>[2x]TIKVGINGFGRIGRIVFRAAQKRSDIEIVAINDLLDADYMAYMLKYDSTHGRFDGTVEVKDGHLIVNGKKIRVTAERDPANLKWDEVGVDVVAEATGLFLTDETARKHITAGAKK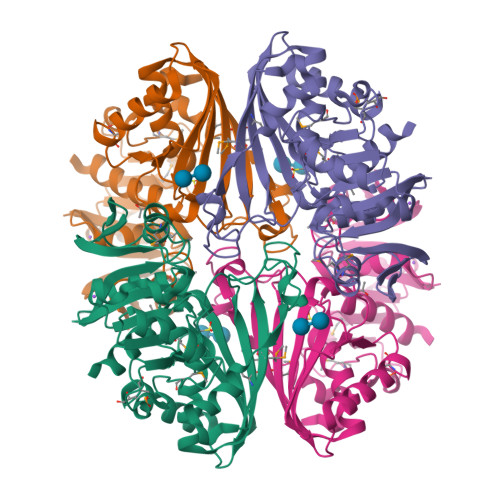VVMTGPSKDNTPMFVKGANFDKYAGQDIVSNASCTTNCLAPLAKVINDNFGIIEGLMTTVHATTATQKTVDGPSHKDWRGGRGASQNIIPSSTGAAKAVGKVLPELNGKLTGMAFRVPTPNVSVVDLTVRLEKAATYEQIKAAVKAAAEGEMKGVLGYTEDDVVSTDFNGEVCTSVFDAKAGIALNDNFVKLVSWYDNETGYSNKVLDLIAHISK>ILDGPYQPTTFTPPTDYWILINSNTNGVVYESTNNSDFWTAVIAVEPHVNPVDRQYNVFGENKQFNVRNDSDKWKFLEMFRGSSQNDFYNRRTLTSDTRLVGILKYGGRIWTFHGETPRATTDSSNTANLNGISITIHSEFYIIPRSQESKCNEYINN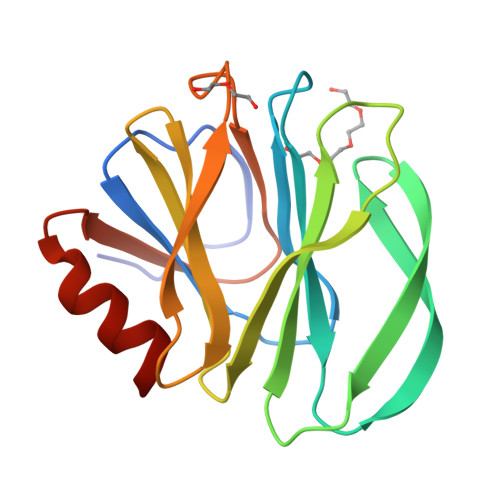GL[3x]> QKWKWWEEERYPEGIKWKFLEHKGPVFAPPYEPLPENVKFYYDGKVMKLSPKAEEVATFFAKMLDHEYTTKEIFRKNFFKDWRKEMTNEEKNIITNLSKCDFTQMSQYFKAQTEARKQMSKEEKLKIKEENEKLLKEYGFCIMDNHKERIANFKIEPPGLFRGRGNHPKMGMLKRRIMPEDIIINCSKDAKVPSPPPGHKWKEVRHDNKVTWLVSWTENIQGSIKYIMLNPSSRIKGEKDWQKYETARRLKKCVDKIRNQYREDWKSKEMKVRQRAVALYFIDKLALRAGNEKEEGETADTVGCCSLRVEHINLHPELDGQEYVVEFDFLGKDSIRYYNKVPVEKRVFKNLQLFMENKQPEDDLFDRLNTGILNKHLQDLMEGLTAKVFRTYNASITLQQQLKELTAPDENIPAKILSYNRANRAVAILCNHQRAP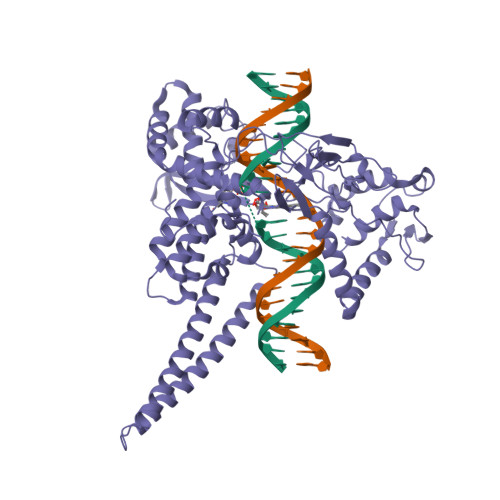PKTFEKSMMNLQTKIDAKKEQLADARRDLKSAKADAKVMKDAKTKKVVESKKKAVQRLEEQLMKLEVQATDREENKQIALGTSKLSYLDPRITVAWCKKWGVPIEKIYNKTQREKFAWAIDMADEDYEF> MTLQNQEFIAGLKAKFAEHRIVFWHDPDKRFLEELDNLELENVTLLDMTDQSQLAVKKRIEIDEPEQQFLLWFPHDAPPKEFDWLLDIRLYSTEFHADFAAITLNTLGIPQLGLREHIQRRKAFFSTKRLSALKGLVTEQENEASLDKKMVAVIAGVKTAKTEEILFSLITQYVNQQKDDDSDLENTLAMLKRHDLEGVLWDILNQEMGYQAEHPTLENLILKLFCTDLSAQADPQKREWLEKNVLATPSGRASALAFMVTWRADRRYKEAYDYCAQQMQDALRPEDQYRLSSPYDLHECETTLSIEQTIIHALVTQLLEESTTLDREAFKKLLSERQSKYWCQTRQEYC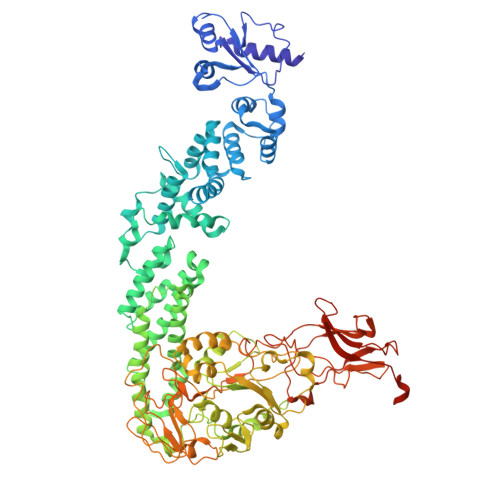AIYDALRQAERLLNLRNRHIDGFHYQDSATFWKAYCEELFRFDQAYRLFNEYALLVHSKGAMILKSLDDYIEALYSNWYLAELSRSWNKVLETENRMQEWRIAGVPRQQNFYNEVVKPQFNNPQIKRVFVIISDALRYEVAEELGNQINTEKRFTAELRSQLGVLPSYTQLGMAALLPHDEICYQPGSGDIVYADGLSTSGTPNRDTILKKYKGMAVKSDDLLKWKNQQGRDLIRDYEVVYIWHNTIDAMGDSASTEEKTFEACRNAVVELKDLVTRVINRLHGTRIIVTADHGFLFQQQPLSGQDKTTLQIKPDNTIKNHKRFIIGHQLPADDFCWKGKVADTAGVSDNSEFLIPKGIQRFHFSGGARFVHGGAMLQEVCVPVLQVKALQKTAAEKQPQRRPVDIVKHHPLIKLVNNIDKVSLLQTHPVGELYEPRTLNIFIVDNANNVVSGKERICFDSDNNTMEKRVRDVTLKLIGANFNRRNEYWLILEDAQTETGYQKYPVIIDLAFQDDFFKETAAAKFERQHMDSSTSAA> GSDILQELLRVSEKAANIARACRQQETLFQLLIEEKKEGEKNKKFAVDFKTLADVLVQEVIKENMENKFPGLGKKIFGEESNELTNDLGEKIIMRLGPTEEETVALLSKVLNGNKLASEALAKVVHQDVFFSDPALDSVEINIPQDILGIWVDPIDSTYQYIKGSADITPNQGIFPSGLQCVTVLIGVYDIQTGVPLMGVINQPFVSQDLHTRRWKGQCYWGLSYLGTNIHSLLPPVSTRSNSEAQSQGTQNPSSEGSCRFSVVISTSEKETIKGALSHVCGERIFRAAGAGYKSLCVILGLADIYIFSEDTTFKWDSCAAHAILRAMGGGMVDLKECLERNPDTGLDLPQLVYHVGNEGAAGVDQWANKGGLIAYRSEKQLETFLSRL

Inositol polyphosphate 1-phosphatase (INPP1) is a prototype member of metal-dependent/lithium-inhibited phosphomonoesterase protein family defined by a conserved three-dimensional core structure. Enzymes within this family function in distinct pathways including inositide signaling, gluconeogenesis, and sulfur assimilation. INPP1 catalyzes the metal-dependent hydrolysis of the phosphomonoester bond from the 1 position phosphate of Ins(1,4)P2 or Ins(1,3,4)P3 to yield inositol 4-phosphate and inositol 3,4-bisphosphate, respectively. Conserved secondary structural elements comprise juxtaposed metal binding pockets and define a shared sequence pattern of D54…E79E80…D153PID156S157T158…D317 as shown for INPP1.

We tested the effects of substrate addition by co-crystallization of INPP1 with a 10X molar excess of Ins(1,3,4)P3 substrate and 2 mM inhibitory Gd3+. Although we could not confidently model the substrate in the resultant structure, metal sites GD1 and GD3 became equivalently occupied. Difference Fourier analysis showed densities peaks of 20.5σ and 20.0σ in metal sites GD1 and GD3, respectively, giving a relative occupancy of 1.0. Consistent with the Fo-Fc differences, anomalous differences peaks of 15.4σ and 14.0σ were calculated, giving a relative occupancy 1.1. Whereas in the absence of substrate, the gadolinium in metal site GD3 were found at half occupancy and had B-factors greater than twice the average, and in the presence of substrate, the gadolinium in site metal site GD3 was well ordered, refined to full occupancy and had B-factors well below the global average. Co-crystallization with Gd3+ but in the presence of substrate (I(1,3,4)P3) resulted in equivalent occupancies of metal sites GD1 and GD3 consistent with the hypothesis that substrate binding alters affinity at metal site GD3 by contributing an additional coordinating ligand through phosphate oxygen. The observation occupancy at a second/third site is also consistent with previous kinetic studies which demonstrated metal binding in INPP1 is cooperative with a Hill co-efficient of 1.9 which predicts if metal site 1 is predominantly bound in the absence of substrate, that an additional two metals are bound cooperatively upon substrate binding. It is noteworthy that the addition of substrate resulted in a significant change in the ratio and intensity of electron density peaks such that metal sites equivalent occupancies of sites GD1 and GD3, each having a tremendous signal exceeding 20 sigma. Anomalous signals confirm this is because of metal binding. In the Gd3+/Ins(1,3,4)P3 and Gd3+/Li+/Ins(1,3,4)P3 structures, the ion could either be a phosphate from the Ins(1,3,4)P3 substrate molecule or a sulfate from the Gd2(SO4)3 in the crystallization solutions. While we did not observe the Ins(1,3,4)P3 substrate, we hypothesize the sulfates and/or phosphates seen in the INPP1 structures represent the 1- and 4-PO4 positions that would be found with ordered substrate or reaction product.>MGAEKKLFLKALKEKFEEDPKEKYTKFYVFGGWRQSARKREFVEAAEKLAEKRGGIPFYNPDIGVPLGQRKLMPYKLSGTDYIVEGDDLHFMNNAAMQQFWDDIRRTVIVGMDTAHAVLEKRLGVEVTPETINEYMETINHALPGGAVVQEHMVEVHPALAWDCYAKIFTGDDELADEIDKKFLIDINKLFPEEQAEQLKAAIGKRTYQVSRVPTLVGRVCDGGTIARWSAMQIGMSFITAYKLCAGEAAIADFSYAAKHADVIQMGTLLPARRARGPNEPGGIPFGILADVVQTTRVSDDPVEQSLEVVASGAMLYDQIWLGSYMSGGVGFTQYATASYTDDILDDFSYYGYDYVEKKYGICGAKPTMDVVEDIATEVTLYALECYDEFPALLEDHFGGSQRAAVAAAASGISVCMATGNSNAGLNGWYLSQILHKEYHSRLGFYGYDLQDQCGASNSLSIRNDESSPLELRGPNYPNYAMNVGHQGEYAGITQAAHSARKDAFALNPLIKVAFADPSLVFDFSHPRKEFARGALREFEPAGERDPIIPAH[2x];>MVKYEDKICLYNAKGELVEENVPLEAISPLYNPTIQKLVKDIKRTVAVNLAGIENALKTGAVGGKACVIPGRTLDLPIVENAETIMEYVDKLLRISPDDDTSVKLINDGKQMAVQLPSKRLEVAAEYSISMLNTAMALKEAIIKTFDVDMFDAPMVHAAIL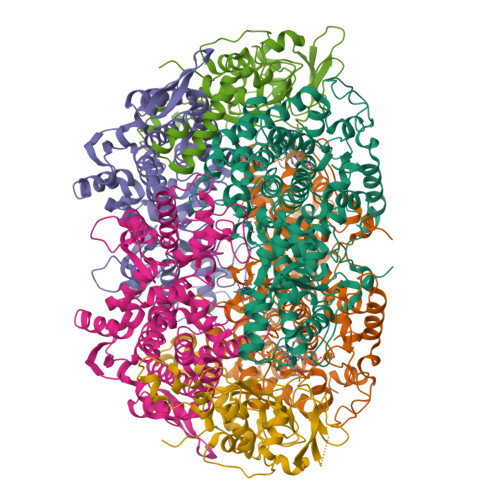GRYPQVPDYMGANIASLLGAPTNLEGLGYALRNIMVNHYVATTKKNIMNAVAFASIMEQTAMFEMGDAIGSFERLHLLGLAYQGLNADNLVIDLVKANGKNGTVGTVVASIVERALEDGVITEDKKMPSGFVLYKPVDVAKWNAYAAAGLVAAVIVNCGAARAAQNVASTILYYNDIIEYETGLPGVDFGRAEGTAVGFSFFSHSIYGGGGPGIFNGNHIVTRHSKGFAIPPVCAAMCVDAGTQMFSPEKTSALVGAVFSAIDEFREPLKYVIDGALAVKDKI[2x];>MAYKPQFYPGETKIAQNRRNHMNPEVELEKLREIPDEDVVKIMGHRQPGEDYKTIHPPLEEMDLPDDYVRDLVEPINGAKEGHRIRYIQFADSMYFAPAQPYDRARTYMWRFRGVDTGTLSGRQVIEMRESDLEALSKNFLIDTAFFDPARCGIRGATVHGHSLRLDENGLMFDALQRYVYDEKTGHVVYVKDQVGRPLDEPVDVGELLPEEKLREITTIYRKDGVPMREDKELLTIVKRIHRARTLGGFCPTEDTFKQL[2x]> GAMAQQPVVRVGEWLVTPSINQISRNGRQLTLEPRLIDLLVFFAQHSGEVLSRDELIDNVWKRSIVTNHVVTQSISELRKSLKDNDEDSPVYIATVPKRGYKLMVPVIWY

One system used by E. coli is the Cad-system, that consists of the cytosolic protein CadA and the membrane proteins CadB and CadC. The pH-receptor CadC senses a drop of the external pH and activates transcription of cadBA below pH 6.64, 5. CadC belongs to the family of ToxR-like receptors. ToxR-like receptors are characterized by a conserved modular composition: external signals are sensed by a periplasmic sensor domain and are transduced through a single transmembrane helix to a cytoplasmic DBD of an OmpR type, which acts as effector domain to regulate gene expression.

To characterize the CadC effector domain and the interaction with DNA, we first determined the crystal structure of the CadC DBD (amino acids 1–107) at 2.0 Å resolution. The overall fold and secondary structure is characteristic for the winged helix-turn-helix (HTH) motif found in members of the OmpR family effector domains. Thus, CadC comprises a recognition helix (α3) and a β-hairpin wing (β5-loop-β6) within a compact fold with the topology β1-β2-β3-β4-α1-α2-α3-β5-β6-β7. To our knowledge, the CadC DBD represents the first structure of a ToxR-like DBD. A unique feature of the CadC DBD is an additional short β-strand (β7) that extends the highly conserved C-terminal β-sheet (β1-β4) in OmpR-type DBDs. Consequently, the β-sheet in CadC is shifted towards the site of the β4 strand to maintain a compact globular fold. The additional strand β7 is important for the structural integrity of CadC, as a truncated variant (CadC1-102) was less soluble and unstable. The highest structural similarity of CadC1-107 with an effector domain bound to DNA is found with PhoB. While SAXS data of CadC1-107 alone are in excellent agreement with the crystal structure (χ2 of 0.98), analysis of the CadC1-107 41-mer Cad1 DNA complex indicates the presence of two domains bound to the cadBA promoter DNA. We have recently shown that the CadC DBD is not per se dimeric. This is confirmed by the monomeric state of the DBD in the crystal and in solution as evidenced by our NMR and SAXS data.>MTKVLYITAHPHDDTQSFSMAVGKAFIDTYKEVNPDHEVETIDLYIEDIPHIDVDVFSGWGKLRSGQGFDQLSSDEKAKVGRLSELCEQFVSADKYIFVSPLWNFSFPPVLKAYIDSVAVAGKTFKYTEQGPVGLLTDKKALHIQARGGIYSEGPAAQMEMGHRYLSIIMQFFGVPSFDGLFVEGHNAMPDKAQEIKEKAVARAKDL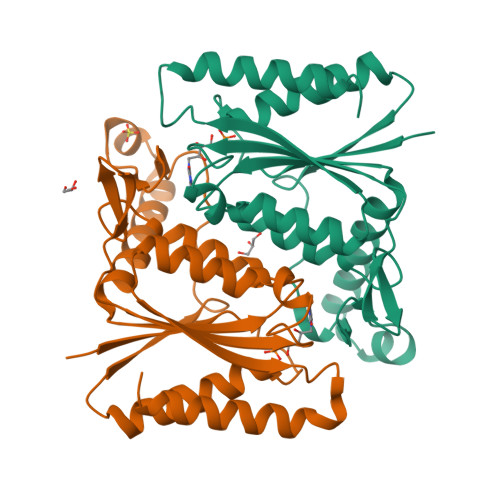AHTF[2x]Here we identify the intracellular NAT16 as the human histidine acetyltransferase (HisAT) responsible for histidine acetylation in vitro and in vivo. Acetylhistidine is synthesized from histidine and acetyl coenzyme A (Ac-CoA) by a histidine acetyltransferase (HisAT, EC:2.3.1.33). We find that HisAT adopts a double-GNAT (Gcn5-related N-Acetyltransferase) fold where the N-terminal domain binds acetyl-CoA and with distinct active site conformation allowing the binding of histidine in between the two domains. Our results indicate that HisAT catalysis occurs via a ternary complex, and the ternary complex is likely stabilized by the oxyanion hole generated by the residues Gly123 and Leu124 of the β-bulge.

The HisAT crystals with CoA disulfide were obtained in the presence of histidine, arginine, and imidazole. Arginine was the amino acid substrate with most activity in the substrate screening without an imidazole side chain. The crystal structure with arginine had the substrate residue occupying a very similar position to histidine. The size of the side chain and the differences in hydrogen bonding disrupted the water chain that was present around the histidine side chain, so that some of the water molecules were displaced or not present. The missing waters could also be explained by the comparatively poorer diffraction quality of this crystal. The substrate binding site combines the preference for aromatic and positively charged amino acid side chains, making histidine the preferred substrate, although we also obtained a crystal structure with arginine in the substrate position. The crystals of the P63 space group invariably contained a CoA disulfide.

> MKLEPEAEAEPLDFVVATEREFEEVLAISGGIYGGLDYLPSRYHSWLRDPDRTVVLAKRNGGVIALESVNVIDAGETVLVEGLRVAPWERGKGVAGLLQRFCSQLVKRQHPGVKVARLTRDDQLGPRELKKYRLITKQGILLVRFNASALLAGLGARLAALRTSGTFSPLPTEAVSEAGGDVARLLLSPSVQRDVLPGGTIIQDWQPYRPSESNLRLLAAKGLEWRVDSRARPRVLTLCTRPFPIPHGGDGTWRYLNIDAFGSDGAQVQSQLLWHLQRQAPRLVGLNVMCQLFLEPQLWSQLADFCQVGLGLELVKGYTEQYLLEADIHHHHHH> TFISRFAPDQPRKGADILVEALERQGVETVFAYPGGASMEIHQALTRSSSIRNVLPRHEQGGVFAAEGYARSSGKPGICIATSGPGATNLVSGLADALLDSVPLVAITGQVPRRMIGTDAFQETPIVEVTRSITKHNYLVMDVEDIPRIIEEAFFLATSGRPGPVLVDVPKDIQQQLAIPNWEQAMRLPGYM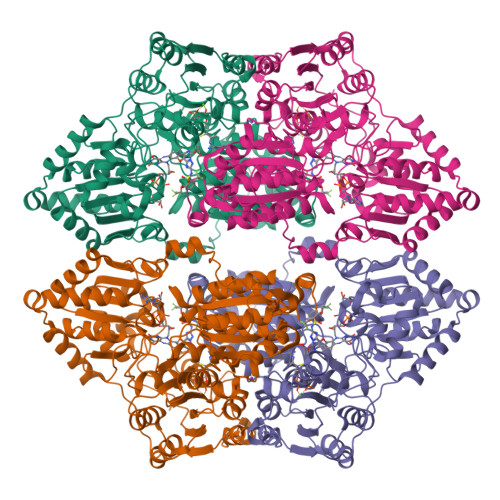SRMPKPPEDSHLEQIVRLISESKKPVLYVGGGCLNSSDELGRFVELTGIPVASTLMGLGSYPCDDELSLHMLGMHGTVYANYAVEHSDLLLAFGVRFDDRVTGKLEAFASRAKIVHIDIDSAEIGKNKTPHVSVCGDVKLALQGMNKVLENRAEELKLDFGVWRNELNVQKQKFPLSFKTFGEAIPPQYAIKVLDELTDGKAIISTGVGQHQMWAAQFYNYKKPRQWLSSGGLGAMGFGLPAAIGASVANPDAIVVDIDGDGSFIMNVQELATIRVENLPVKVLLLNNQHLGMVMQWEDRFYKANRAHTFLGDPAQEDEIFPNMLLFAAACGIPAARVTKKADLREAIQTMLDTPGPYLLDVICPHQEHVLPMIPSGGTFNDVITEGDGRLEHHHHHH6-[(2R)-oxiran-2-yl]-L-norleucine | C8 H15 N O3 | 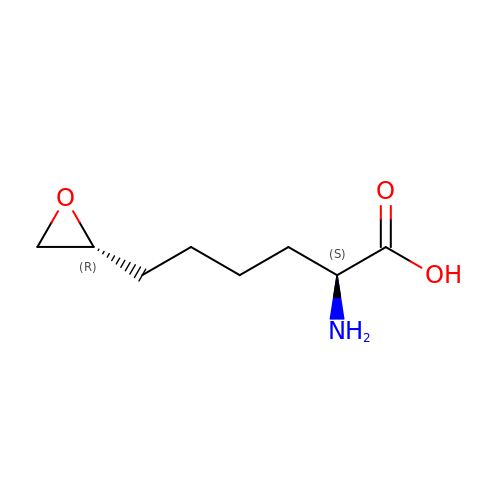VESDHWISIJZIDY-RQJHMYQMSA-N>GSPRVVVIKKGSNGYGFYLRAGPEQKGQIIKDIEPGSPAEAAGLKNNDLVVAVNGKSVEALD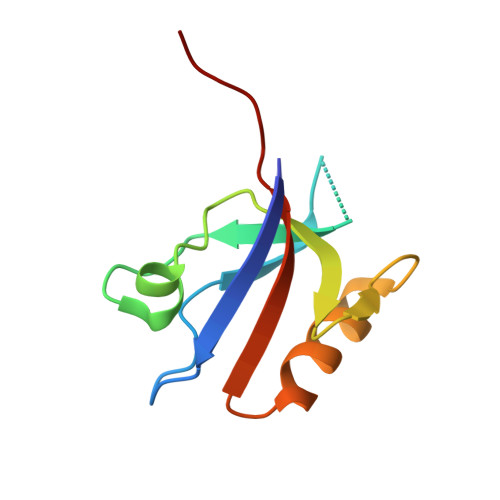HDGVVEMIRKGGDQTTLLVLDKQEAKL[2x]>[2x]ARDPKHDILFEPIQIGPKTLRNRFYQVPHCIGAGSDKPGFQSAHRSVKAEGGWAALNTEYCSINPESDDTHRLSARIWDEGDVRNLKAMTDEVHKYGALAGVELWYGGAHAPNMESRATPRGPSQYASEFETLSYCKEMDLSDIAQVQQFYVDAAKRSRDAGFDIVYVYGAHSYLPLQFLNPYYNKRTDKYGGSLENRARFWLETLEKVKHAVGSDCAIATRFGVDTVYGPGQIEAEVDGQKFVEMADSLVDMWDITIGDIAEWGEDAGPSRFYQQGHTIPWVKLVKQVSKKPVLGVGRYTDPEKMIEIVTKGYADIIGCARPSIADPFLPQKVEQGRYDDIRVCIGC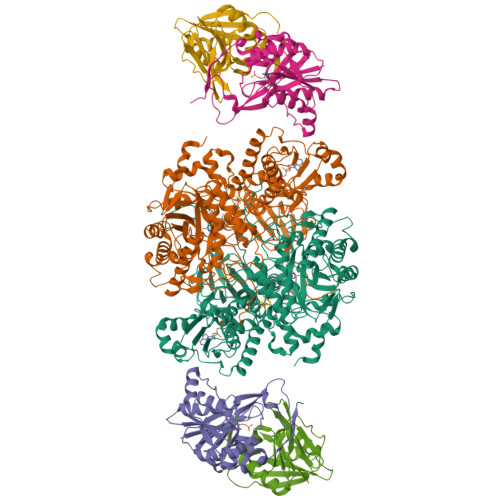NVCISRWEIGGPPMICTQNATAGEEYRRGWHPEKFRQTKNKDSVLIVGAGPSGSEAARVLMESGYTVHLTDTAEKIGGHLNQVAALPGLGEWSYHRDYRETQITKLLKKNKESQLALGQKPMTADDVLQYGADKVIIATGARWNTDGTNCLTHDPIPGADASLPDQLTPEQVMDGKKKIGKRVVILNADTYFMAPSLAEKLATAGHEVTIVSGVHLANYMHFTLEYPNMMRRLHELHVEELGDHFCSRIEPGRMEIYNIWGDGSKRTYRGPGVSPRDANTSHRWIEFDSLVLVTGRHSECTLWNELKARESEWAENDIKGIYLIGDAEAPRLIADATFTGHRVAREIEEANPQIAIPYKRETIAWGTPHMPGGNFKIEYKV;>MKILVAVKQTAALEEDFEIREDGMDVDEDFMMYDLNEWDDFSLEEAMKIKESSDTDVEVVVVSVGPDRVDESLRKCLAKGADRAVRVWDDAAEGSDAIVVGRILTEVIKKEAPDMVFAGVQSSDQAYASTGISVASYLNWPHAAVVADLQYKPGDNKAVIRRELEGGMLQEVEINCPAVLTIQLGINKPRYASLRGIKQAATKPIEEVSLADIGLSANDVGAAQSMSRVRRMYIPEKGRATMIEGTISEQAAKIIQIINEFKGA[2x];>SKILVIAEHRRNDLRPVSLELIGAANGLKKSGEDKVVVAVIGSQADAFVPALSVNGVDELVVVKGSSIDFDPDVFEASVSALIAAHNPSVVLLPHSVDSLGYASSLASKTGYGFATDVYIVEYQGDELVATRGGYNQKVNVEVDFPGKSTVVLTIRPSVFKPLEGAGSPVVSNVDAPSVQSRSQNKDYVEVGGGNDIDITTVDFIMSIGRGIGEETNVEQFRELADEAGATLCCSRPIADAGWLPKSRQVGQSGKVVGSCKLYVAMGISGSIQHMAGMKHVPTIIAVNTDPGASIFTIAKYGIVADIFDIEEELKAQLAA[2x]>[4x]MVAVEQSEASRLGPVFDSCRANNRAALIGYLPTGYPDVPASVAAMTALVESGCDIIEVGVPYSDPGMDGPTIARATEAALRGGVRVRDTLAAVEAISIAGGRAVVMTYWNPVLRYGVDAFARDLAAAGGLGLITPDLIPDEAQQWLAASEEHRLDRIFLVAPSSTPERLAATVEASRGFVYAASTMGVTGARDAVSQAAPELVGRVKAVSDIPVGVGLGVRSRAQAAQIAQYADGVIVGSALVTALTEGLPRLRALTGELAAGVRLGMSAHHHHHH;>[4x]MSAAIAEPTSHDPDSGGHFGGPSGWGGRYVPEALMAVIEEVTAAYQKERVSQDFLDDLDRLQANYAGRPSPL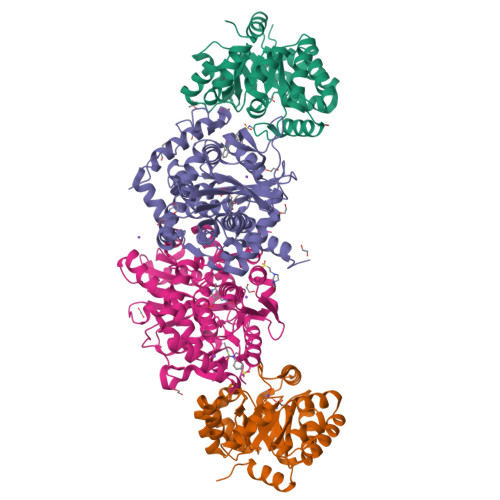YEATRLSQHAGSARIFLKREDLNHTGSHKINNVLGQALLARRMGKTRVIAETGAGQHGVATATACALLGLDCVIYMGGIDTARQALNVARMRLLGAEVVAVQTGSKTLKDAINEAFRDWVANADNTYYCFGTAAGPHPFPTMVRDFQRIIGMEARVQIQGQAGRLPDAVVACVGGGSNAIGIFHAFLDDPGVRLVGFEAAGDGVETGRHAATFTAGSPGAFHGSFSYLLQDEDGQTIESHSISAGLDYPGVGPEHAWLKEAGRVDYRPITDSEAMDAFGLLCRMEGIIPAIESAHAVAGALKLGVELGRGAVIVVNLSGRGDKDVETAAKWFGLLGND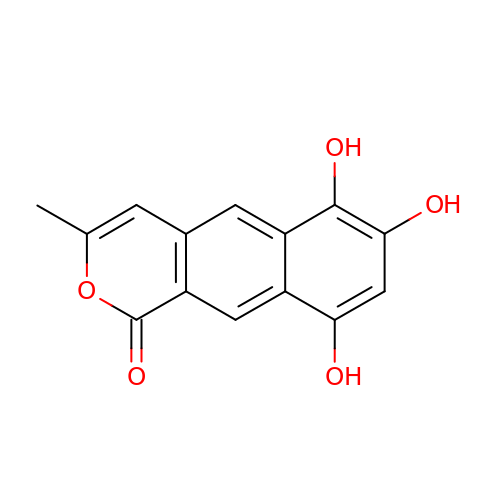6,7,9-trihydroxy-3-methyl-1H-benzo[g]isochromen-1-one | C14 H10 O5 | JSPFABGVYLULRJ-UHFFFAOYSA-N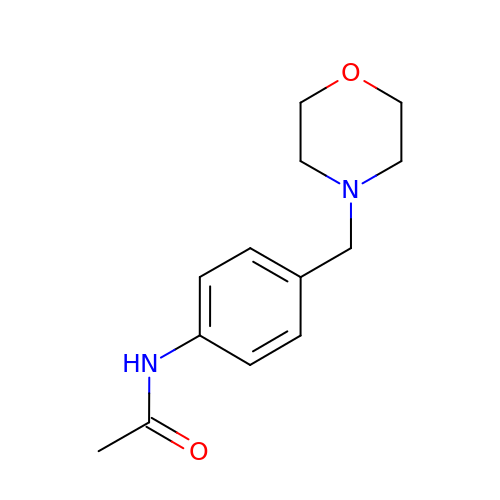N-{4-[(morpholin-4-yl)methyl]phenyl}acetamide | C13 H18 N2 O2 | KFRGDVNNAPFDCF-UHFFFAOYSA-N> MGSSHHHHHHSSGLVPRGSHAGAAASDSKGAEISGAGASFIYPLVSKWSADYNAATGNKVNYQSIGSGGGIAQIKAGTVDFGSTDKPLDSAELQQAGLGQFPSAIGGVVPVVNLEGIAPGKLRLTGALLGDIFLGKVTMWNDAAIVAANP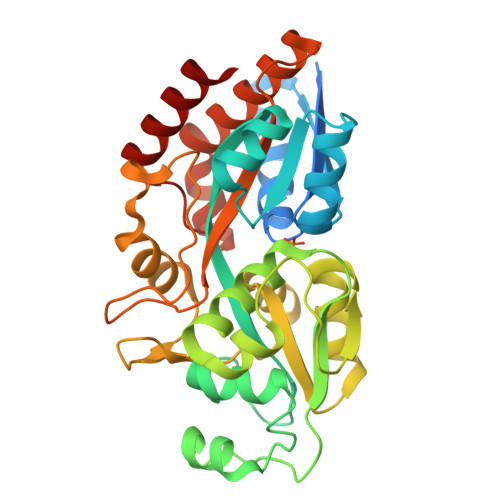GVTLPATKINLVHRSDGSGTTFNFSNYLSKVSPEWKSKVGEGTSVQWPGGVGGKGNEGVASYVQQIKGSIGYVELAYALQNKMPYTSLQNAAGQWIEPNAESFAAAAASADWANARDFNLVITNAPGEKAWPITATNFMLMHKQPKDAARSKATLDFFKWALENGQAQASELHYVPLPPELVKQIEAYWGSEFK L-Methionine Tenofovir | C14 H23 N6 O5 P S | 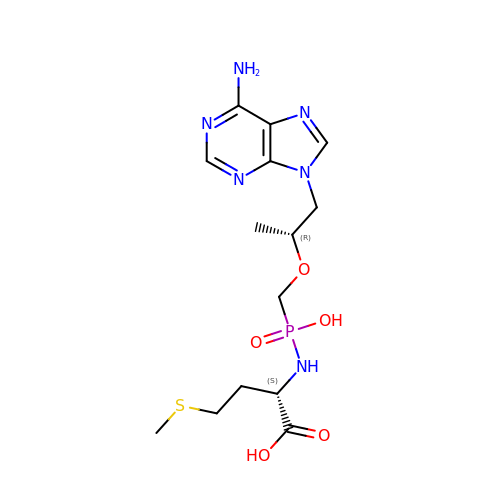PEQPYHOXTFLJCT-ZJUUUORDSA-N> AVKYYTLEEIQKHNNSKSTWLILHYKVYDLTKFLEEHVGGEEVLREQAGG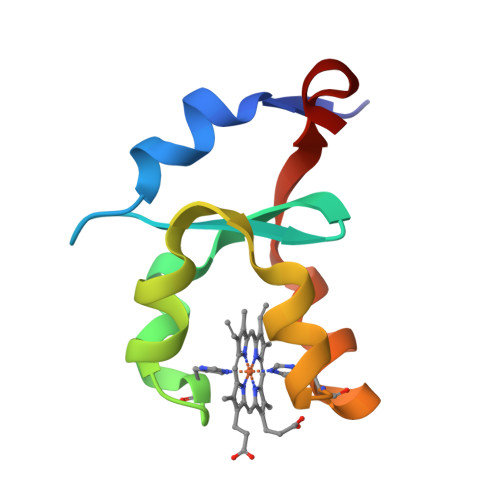DATENFEDVGHSTDARELSKTFIIGELHPDDR> MWVDFIDQTKSLKVSVNNYFYYLDRIKKLFTYLNDLRKHILKKYVYTINHKRIAINYLYFSMVTGLSGAALATMIRLELAHPGSPFFKGDSLRYLQVVTAHGLIMVFFVVVPILFGGFANFLIPYHVGSKDVAYPRLNSIGFWIQPCGYILLAKIGFLRPQFWRYYDKTSFSFPFLEKMKYNQYKEYKNDYLFYLDFLKKEITDDHSFFWKARKVIKLPQYSVFSFVPLKLMMWKTMINYPESFWYAASRVVQSRRKKVFVTKCSARTLTTAGWTFITPFSSNIKYTGVGSQDILILSVVFAGISTTISFTNLLITRRTLAMPGLRHRRVLMPFVTISIFLTLRMLATITPVLGAAVIMMAFDRHWQTTFFEYAYGGDPILSQHLFWFFGHPEVYVLIIPTFGFINMIVPHNNTRRVASKH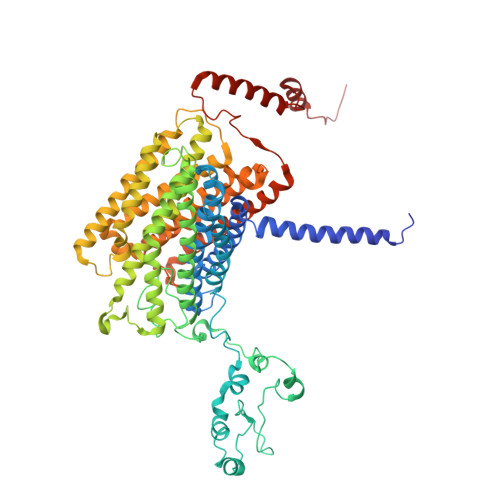HMIWAIYVMAYMGYLVWGHHMYLVGLDHRSRTMYSTITIMISMPATIKVVNWTLSLVNGALKIDLPFLFSMSFLLLFLVAGFTGMWLSHVSLNVSMHDTFYVVAHFHIMLSGAAMTGIFSGIYYYFNALFGVKYSRMFGYMHLIYYSGGQWVAFVPLFYLGFSGMPRRIHDYPVVFMGWHSMSTTGHFITLVGIIFFFLMMFDSHIERRASTSTTLGLPRWYKRISYYIFKIRYLQHTKSKMNGIPGSTVRLMLINRHFVEYEVYEK> 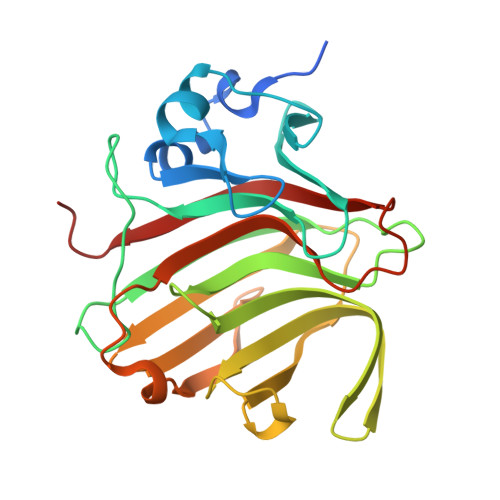MNSLLTLSLLATNAMFLTAVSSIDTFLPVLNEAKLQWPTSALAASSEELLGGYVGSQFYLQDGKYMQFQIAGSSNRCELRQMIPDGGSEIGWAVDDGTTHTATSSIVVPEQVDGVEEVTIMQIHSGEAPQLRISWIRSKSLDGVAYEDFIMSTVRIGTGDSSDNFVKTHLADRTAGAMSFQIDVKDSKLTITVNGNVVVNGQDLSFWDGTDSCYFKAGAYNNNPTSESATARIKFAALAWVDHHHH> CLLCFTTYSERLRICQMFVGMRSPKLEECEEAFTAAFQGLSDTEINYDERSHLHDTFTQMTHALQELAAAQGSFEVAFPDAAEKMKKVITQLKEAQACIPPCGLQEFARRFLCSGCYSRVCDLPLDCPVQDVTVTRGDQAMFSCIVNFQLPKEEITYSWKFAGGGLRTQDLSYFRDMPRAEGYLARIRPAQLTHRGTFSCVIKQDQRPLARLYFFLNVTGLVPRGSHHHHHHHHHH

SPACA6 is a sperm-expressed surface protein that is critical for gamete fusion during mammalian sexual reproduction. We elucidated the crystal structure of the SPACA6 ectodomain at 2.2-Å resolution, revealing a two-domain protein containing a four-helix bundle and Ig-like β-sandwich connected via a quasi-flexible linker. This structure is reminiscent of IZUMO1, another gamete fusion-associated protein, making SPACA6 and IZUMO1 founding members of a superfamily of fertilization-associated proteins, herein dubbed the IST superfamily. The IST superfamily is defined structurally by its distorted four-helix bundle and a pair of disulfide-bonded CXXC motifs.

We expressed the extracellular domain of human SPACA6 (residues 27–246) in Drosophila S2 cells and purified the protein using nickel-affinity, cation-exchange, and size-exclusion chromatographies. The SPACA6 ectodomain was crystallized using a random matrix microseeding approach, yielding a 2.2-Å resolution dataset. The structure was determined using a combination of fragment-based molecular replacement and SAD phasing data from bromide soaks, with the final refined model consisting of residues 27–246. The SPACA6 ectodomain, with dimensions of 20 Å × 20 Å × 85 Å, is made up of seven helices and nine β-strands and adopts an elongated tertiary fold stabilized by six disulfide bonds. The 4HB domain of SPACA6 includes four main helices (Helices 1–4) arranged in a coiled-coil fashion that alternate between antiparallel and parallel interactions. A small additional single-turn helix (Helix 1′) packs perpendicularly with the bundle, forming a triangular shape with Helices 1 and 2. The core accommodates a disulfide bond between Cys41 and Cys55, which pinches Helices 1 and 2 together at the top, accentuating the triangular shape. Two additional disulfide bonds are formed between the CXXC motif of Helix 1’ and another CXXC motif found at the tip of a β-hairpin in the hinge region. A network of covalent and electrostatic contacts in the hinge region appear to stabilize the orientation between the 4HB and Ig-like domains. In contrast, the helical bundle in SPACA6 has an approximately 10° lean in the opposite direction.> MNSEYDYLFKLLLIGNSGVGKSCLLLRFSDDTYTNDYISTIGVDFKIKTVELDGKTVKLQIWDTAGQERFRTITSSYYRGSHGIIIVYDVTDQESF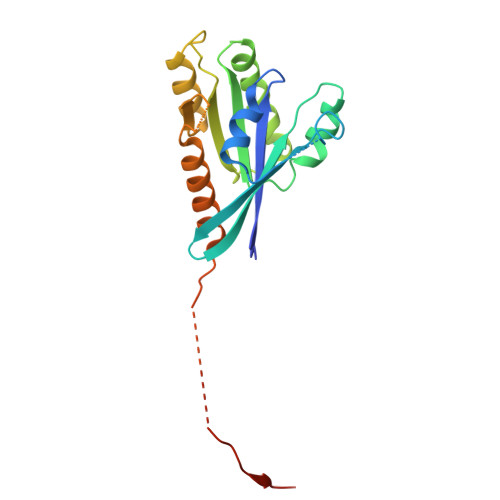NGVKMWLQEIDRYATSTVLKLLVGNKCDLKDKRVVEYDVAKEFADANKMPFLETSALDSTNVEDAFLTMARQIKESMSQQNLNETTQKKEDKGNVNLKGQSLTNTGGGCC>[4x]ATILVVTGTGTGVGKTVVCAALASAARQAGIDVAVCKPVQTGTARGDDDLAEV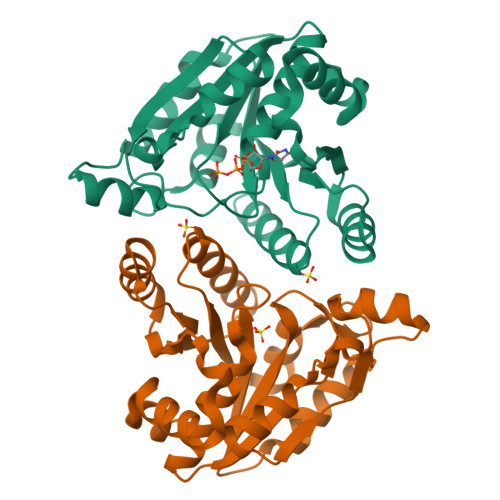GRLAGVTQLAGLARYPQPMAPAAAAEHAGMALPARDQIVRLIADLDRPGRLTLVEGAGGLLVELAEPGVTLRDVAVDVAAAALVVVTADLGTLNHTKLTLEALAAQQVSCAGLVIGSWPDPPGLVAASNRSALARIAMVRAALPAGAASLDAGDFAAMSAAAFDRNWVAGLV>[2x]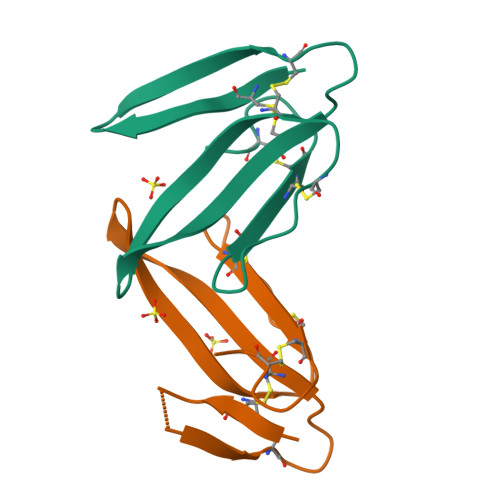LTCVTDKSFGGVITEECAAGQKICFKNWKKMGPKLYDVKRGCTATCPKADDNGCVKCCNTDKCNK> MLKREMNIADYDAELWQAMEQEKVRQEEHIELIASENYTSPRVMQAQGSQLTNKFAEGYPGKRYYGGCEYVDIVEQLAIDRAKELFGADYANVQPHSGSQANFAVYTALLEPGDTVLGMNLAHGGHLTHGSPVNFSGKLYNIVPYGIDATGHIDYADLEKQAKEHKPKMIIGGFSAYSGVVDWAKMREIADSIGAYLFVDMAHVAGLVAAGVYPNPVPHAHVVTTTTHKTLAGPRGGLILAKGGSEELYKKLNSAVFPGGQGGPLMHVIAGKAVALKEAMEPEFKTYQQQVAKN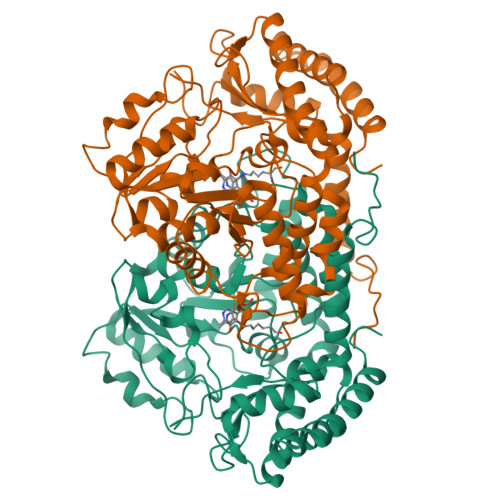AKAMVEVFLERGYKVVSGGTDNHLFLVDLVDKNLTGKEADAALGRANITVNKNSVPNDPKSPFVTSGIRVGTPAITRRGFKEAEAKELAGWMCDVLDSINDEAVIERIKGKVLDICARYPVYA> MSVVLPVAKRGEDILKLIAAPVSANELNSNWLYQLA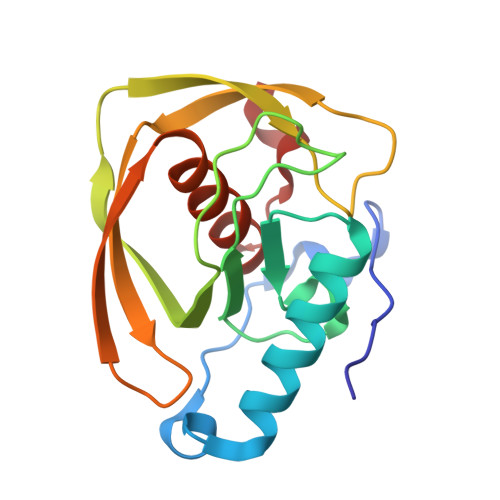DAMHATMLERNGVGIAAPQVYISKRVIIVASRPNPRYPDAPEMNAVVMVNPEILEFSSEMCLGEEGCLSVPDERGQVERAEMVKVKYLTLQGEMVETVFQGFPARIVQHEVDHLNGILFVERIS1-[(7-carbamimidoylnaphthalen-2-yl)methyl]-6-({1-[(1Z)-ethanimidoyl]piperidin-4-yl}oxy)-2-(propan-2-yl)-1H-indole-4-carboxylic 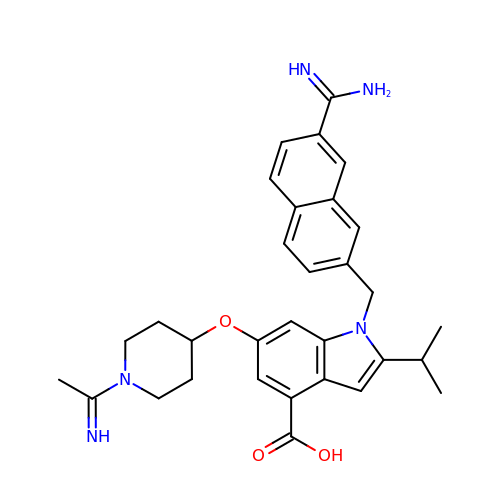acid | C31 H35 N5 O3 | WBDOXNXLJBVELO-UHFFFAOYSA-N1-(2-CHLOROBENZYL)-4-HEXYLPYRIDIN-2(1H)-ONE | C18 H22 Cl N O | 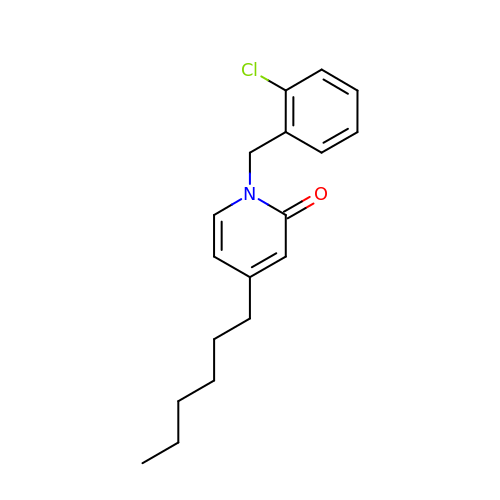PJBRBZYHOXOPFM-UHFFFAOYSA-N>AKLGSVYTEGGFVEGVNKKLSLFGDSIDIFKGIPFAAAPKALEKPERHPGWQGTLKAKSFKKRCLQATLT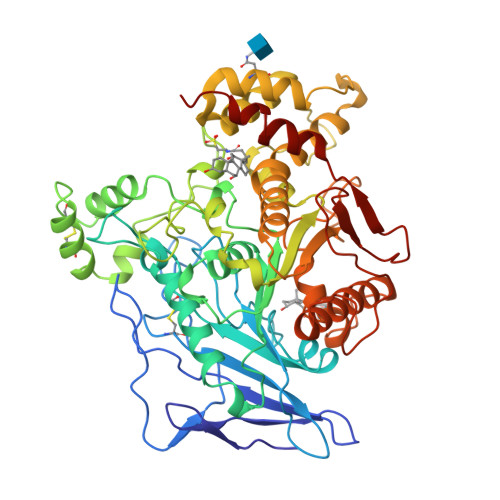QDSTYGNEDCLYLNIWVPQGRKEVSHDLPVMIWIYGGAFLMGASQGANFLSNYLYDGEEIATRGNVIVVTFNYRVGPLGFLSTGDSNLPGNYGLWDQHMAIAWVKRNIEAFGGDPDNITLFGESAGGASVSLQTLSPYNKGLIKRAISQSGVGLCPWAIQQDPLFWAKRIAEKVGCPVDDTSKMAGCLKITDPRALTLAYKLPLGSTEYPKLHYLSFVPVIDGDFIPDDPVNLYANAADVDYIAGTNDMDGHLFVGMDVPAINSNKQDVTEEDFYKLVSGLTVTKGLRGANATYEVYTEPWAQDSSQETRKKTMVDLETDILFLIPTKIAVAQHKSHAKSANTYTYLFSQPSRMPIYPKWMGADHADDLQYVFGKPFATPLGYRAQDRTVSKAMIAYWTNFARTGDPNTGHSTVPANWDPYTLEDDNYLEINKQMDSNSMKLHLRTNYLQFWTQTYQALPTV[2x]>ASMTGGQQMGAPITAYAQQTRGLLGCIITSLTGRDKNQVEGEVQIVSTATQTFLATCINGVCWTVYHGAGTRTIASPKGPVIQMYTNVDQDLVGWPAPQGSRSLTPCTCGSSDLYLVTRHADVIPVRRRGDSRGSLLSPRPISYLKGSSGGPLLCPAGHAVGLFRAAVCTRGVTKAVDFIPVENLETTMRGSHHHHHH[2x];>KKGSVVIV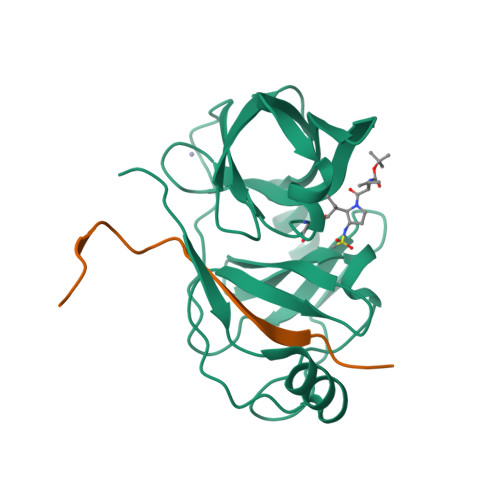GRIVLSGKPAIIPKK[2x]> MRSGRKLGCFTNRLRLPFFSPCSQITALTASHRCKSYVLKFLRGQLPEDLKDVNGALGCLYGTLPDVDEFGQFVISPDVVNSFHQFGYVKMPIPVLDHQQIDKLADEVNELANNVEHHPKTERLYATSLADLTGGPLFFCQGQWRAAWGMHDLIYLPTITVAASQILNNSLVRLWYDEVFMKAARTGPCVPWQQNYARWQHTKPVNHVTVMIALDTMNKDRGAPCLVPGSHRWREGGLLPPVSYDPTKDEAHQLNT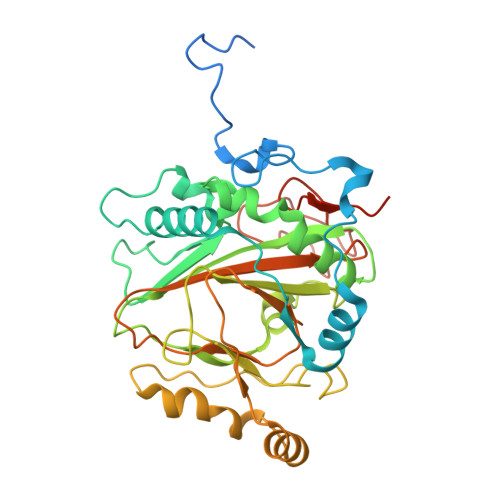IWEIINEEEGEMLMDTPPVTVDLRRGEALLIHPLTLFATHGNRSLDAVRCCFIHYMGEKTYAVQNGPLLPHTTKFQADAMIQGPFYPVVFDPAMTEELTMLPTAPSEEEA[2-(1~{H}-indol-3-yl)ethylamino]phosphonic acid | C10 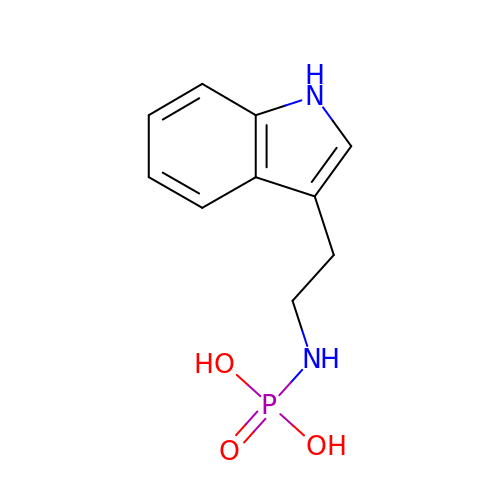H13 N2 O3 P | LZBMOXGGHSGOHA-UHFFFAOYSA-N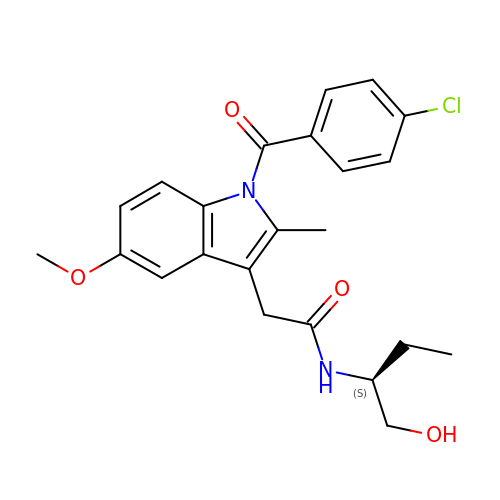2-[1-(4-CHLOROBENZOYL)-5-METHOXY-2-METHYL-1H-INDOL-3-YL]-N-[(1S)-1-(HYDROXYMETHYL)PROPYL]ACETAMIDE | C23 H25 Cl N2 O4 | GKJWXEORYGBJFS-KRWDZBQOSA-N> SAGNDSLPFENIQGDILVGMKKDKEKFVFFHINNATAFKSVLKTYAPANITSVATIIGPVANQPLAFVNLAFSHAGFGALNVTDDLQDTAFSDGQFKDSPNLGDDTSTWEEAFKGTNVDGVFLIGSNDESITAQYRDDLNAKFGDAWTIVYDLDSAARPGNEKGHEHFGYLDGISNPTIPGFGTPHPGQAVVDPGIIFTGRSKDPVMNRPSWALDGSFLVFRKLKQLVPEFNKYVLDNALQNQAGNLTVEEGAELLGSRMFGRWKSGAPIDLSPDFDDPALGNDIERNNNFNYSHPGSDLATDQTRCPFTAHIRKTNPRDLEGQGLFGDTFHAIRAGTPYGPEVTDYEASSNTTTIDRGLAFVEYQSVIGNGFRFQQQAWANNPRFPFSKGPSIQLGLDPVIGQGSPRETFGLDPRNASESFTVPQVIISNGGEYFFSPSITAIVEKFAALEHHHHHH

Dye-decolorizing peroxidases (DyPs) represent a novel family of heme peroxidases that use H2O2 as the final electron acceptor to catalyze the oxidation of various organic compounds. Unlike the crystal structures of fungal class II heme peroxidases, such as lignin peroxidases (LiPs; EC 1.11.1.14), manganese peroxidases (MnPs; EC 1.11.1.13) and versatile peroxidases (VPs; EC 1.11.1.16), DyPs exhibit a unique tertiary structure: (I) DyPs have two domains, composed of α-helix and β-sheet, to form the α/β barrel structure, which is vastly different from the α-helix-rich structure of fungal class II heme peroxidases; (II) the heme molecule binds to the C-terminal region of DyPs protein. In addition, a conserved acidic amino acid (usually aspartic acid) was found in the heme distal region, which is also different from the distal conserved histidine in fungal class II heme peroxidases. However, unlike H2O2, some sterically bulky substrates, such as anthraquinone and azo dyes, are unable to gain access to the heme cavity of a DyP, which means that the oxidation site in DyPs is more likely to localize on the enzyme surface.

The final model of Il‑DyP4 includes one protein monomer (residues 6–450), one heme molecule, one oxygen molecule and 431 water molecules. One heme with an iron is located between the two domains, namely the proximal N- and the distal C-terminal domain. Channel 1 has a length of 15.6 Å, and is located over the heme plane, which is the main channel leading from the protein surface to the heme distal cavity. Another heme access-channel, namely channel 2, from the protein surface leads to the heme propionate with a length of about 7.8 Å. In the heme active center, the side chains of Asp172, Arg335, Leu360 and Phe362 constructed a pocket structure which allows the conversion of H2O2 into H2O in the distal region of Il‑DyP4. Meanwhile, Il‑DyP4 also has a histidine (His312), coordinated to the heme iron as the fifth ligand at a distance of 2.2 Å, which is the same as another heme peroxidases. The conserved GXXDG motif in Il‑DyP4 is shown in Fig. 3b, which consisted of Gly169, Tyr170, Leu171, Asp172 and Gly173. However, the crystal structure of Il‑DyP4 showed that W264 is far away from the proximal conserved histidine residue (H312) (~ 10.4 Å). W380 is located in an extremely hydrophobic environment with five hydrophobic phenylalanines surrounding it, which might facilitate surface interactions between W380 and the substrates that are rich in aromatic moieties, such as dyes.>[6x]GSIAPYLVKIIDPDYEKNERTRIKAQENLRRIRRKQIAEKGDNEDGTDDPSRRRKIDDLVLNEYENQVALEVVAPEDIPVGFNDIGGLDDIIEELKETIIYPLTMPHLYKHGGALLAAPSGVLLYGPPGCGKTMLAKAVAHESGASFINLHISTLTEKWYGDSNKIVRAVFS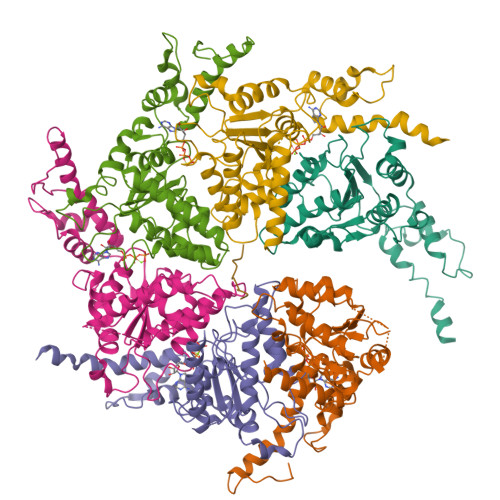LAKKLQPSIIFIDQIDAVLGTRRSGEHEASGMVKAEFMTLWDGLTSTNASGVPNRIVVLGATNRINDIDEAILRRMPKQFPVPLPGLEQRRRILELVLRGTKRDPDFDLDYIARVTAGMSGSDIKETCRDAAMAPMREYIRQHRASGKPLSEINPDDVRGIRTEDFFGRRGGKILSEIPPRQTGYVVQSKNSSEGGYEEVEDDDEQGTAST> MKQGLQLRLSQQLAMTPQLQQAIRLLQLSTLELQQELQQALESNPLLEQTDLHDEVEAKEVEDRESLDTVDALEQKEMPDELPLDASWDEIYTAGTPSGNGVDYQDDELPVYQGETTXXXXXXXXXXXXXXXXXXXXXXXXXXXXXXXXXXQTLQDYLMWQVELTPFTDTDRAIATSIVDAVDDTGYLTIQIEDIVDSIGDDEIGLEEVEAVLKRIQRFDPVGVAAKDLRDCLLIQLSQFA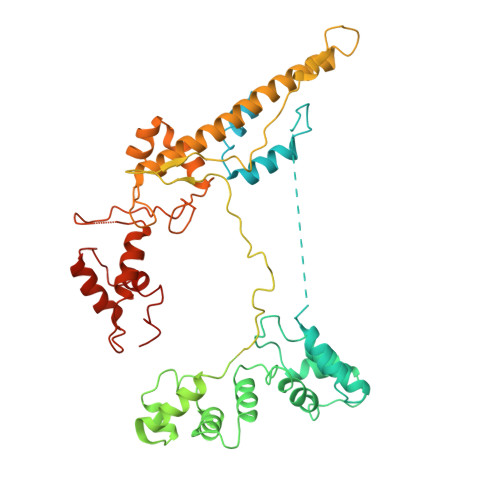KETPWLEEARLIISDHLDLLANHDFRTLMRVTRLKEEVLKEAVNLIQSLDPRPGQSIHTSEPEYVIPDVLVRKVSGRWTVELNADSIPRLKINQQYAAXXXXXXXXXXXXXXXXXXXXXXXXXXXXXXXXXXXXXXXXXXXXXXMGNSARNDADGQFIRSNLQEARWLIKSLESRNDTLLRVSRCIVEQQQAFFEQGEEYMKPMVLADIAQAVEMHESTISRVTTQKYLHSPRGIFELKYFFSSHVNTEGGGEXXXXXXXXXXXXXXXXASSTAIRALVKKLIAAENPAKPLSDSKLTSMLSEQGIMVARRTVAKYRESLSIPPSNQRKQLV>[2x]MKIAVIGQSLFGQEVYKELKNEGHMIVGVFTIPDKDGKVDPLAIEAEKDGVPVFKFPRWRLKGKAITEVVDQYKAVGAELNVLPFCSQFIPMEVIDHPKHGSIIYHPSLLPRHRGASAINWTLIHGDKKGGFTVFWADDGLDTGPILLQRECDVEPNDNVNSIYKRFLFPEGVKGMVEAVRLIATGKAPRIKQPEEGATYECIQKKENSKIDWNQPAEAIHNWIRGNDRVPGAWAEIDGKSVSFYGSTLLENDHFSSNGQPLEIPGASRAALVTKNGLVLFGNDGKMLLVKNLQFEDGKMIPGSQYFKAGVEHHHHHH

10-Formyltetrahydrofolate dehydrogenase (FDH), which is composed of a small N-terminal domain (Nt-FDH) and a large C-terminal domain, is an abundant folate enzyme in the liver and converts 10-formyltetrahydrofolate (10-FTHF) to tetrahydrofolate (THF) and CO2. Nt-FDH alone possesses a hydrolase activity, which converts 10-FTHF to THF and formate in the presence of β-mercaptoethanol. The N-terminal hydrolase domain of FDH (Nt-FDH) binds folate and is homologous to glycinamide ribonucleotide formyltransferase (GART) and methionyl-tRNA formyltransferase (FMT), enzymes that are crucial for de novo purine biosynthesis and translation initiation, respectively. In this study, we determined crystal structures of zebrafish wild-type apo Nt-FDH (zNt-FDH) and its ternary complexes with the substrate 10-formyl-5,8-dideazafolate (10-FDDF) and the products tetrahydrofolate (THF) and formate.

The space group of this THF complex was transformed from the P21212 space group of the apo form, containing one zNt-FDH molecule in the asymmetric unit, to P212121 with two molecules in the asymmetric unit. The structure of each monomer in the THF-bound form of zNt-FDH is nearly identical to the apo form, with an r.m.s.d. of 0.65 Å for 308 Cα atoms; the central hole has a solvent-accessible pocket of similar size in the structures of both apo Nt-FDH and the THF complex. The structure of THF is complete, in contast to that of the human structure, in which only 6-formyltetrahydropterin was observed, providing complete information on the inter­action between THF and its surrounding residues. The pteridine ring of THF is buried in the central cavity and makes a stacking interaction with the side chain of Phe89. The pteridine moiety of THF is recognized by the main-chain carbonyl groups of Gln88, Ile90, Asp138 and Gly140 and the amide group and OD1 atom of Asp142 through direct hydrogen bonds and by the main-chain amide or carbonyl of Asp138, Gly140, Thr143 and Gly144, the OD1 atom of Asp138 and the OG1 atom of Thr143 through water-mediated hydrogen bonds. The hydroxyl O atom of Tyr200 exhibits direct and water-mediated interactions with the O atom of the pABA moiety within each monomer of the dimer, whereas the main-chain atoms of Ala116, Glu201 and Ile203 interact indirectly through water molecules with the O atom of the pABA within a hydrogen-bond distance. In the structure of THF-bound zNt-FDH, the aromatic ring of Tyr200 is observed to rotate by 90° to make space for product binding. An additional potential THF binding site is identified in the cavity between two zNt-FDH molecules, which might contribute to the properties of product inhibition and THF storage reported for FDH. The average B factor (52 Å2) of the THF in the cleft near the interface between two zNt-FDH molecules is greater than that of the THF in the active site (32 Å2), suggesting relatively weak binding of the second THF molecule.> MKHHHHHHMKQNSPLDEENLTQENQDRGTHVDRGLASANVDFAFSLYKQLVLKAPDKNVIFSPVSISTALAFLSLGAHNTTLTEILKGLKFNLTETSEAEIHQSFQHLLRTLNQSSDELQLSMGNAMFVKEQLSLLDRFTEDAKRLYGSEAFATDFQDSAAAKKLINDYVKNGTRGKITDLIKDLDSQTMMVLVNYIFFKAKWEMPFDPQDTHQSRFYLSKKKWVMVPMMSLHHLTIPYFRDEELSCTVVQLNYTGNASVFFILPDQDKMEEVEAMLSRETLARWGDSLEFREIGELYLPKFSISRDYNLNDILLQLGIEEAFTSKADLSGITGARNLAVSQVVHKAVLDVFEEGTEASAATAVKI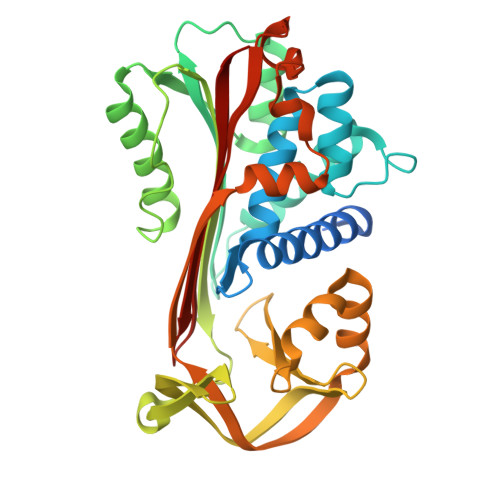TLL Tyrosyl-DNA phosphodiesterase 2 (TDP2) {also known as TRAF and TNF receptor-associated gene (TTRAP) or ETS1-associated protein II (EAPII) } is a 5′-tyrosyl DNA phosphodiesterase that can remove the covalently-attached abortive complexes generated by DNA topoisomerase II (TOP2) when it is unable to complete its normal catalytic cycle. Fortunately, this type of DNA lesion is efficiently repaired, in part though the action of TDP2, which hydrolyses the phosphotyrosyl bond in a magnesium cofactor-dependent reaction, leaving ligatable 5′-phosphate moieties. Consequently, TDP2 has attracted interest as a target for small molecule inhibitors that might have utility in overcoming innate or acquired resistance to TOP2 poisons. Using a ‘humanized’ mouse TDP2 expression construct, we have now determined X-ray crystal structures of the catalytic domain of TDP2 in complex with deazaflavin inhibitors, revealing the unusual molecular interactions underpinning their mode of action.

We therefore created the expression construct m2hTDP2CAT (m2h=mouse-‘to’-human) by mutating the following mouse residues to their human equivalent: E242G, Q278R, Y321C and H323L. We were successful in obtaining diffracting crystals of 148 in complex with m2hTDP2CAT, determining the structure at a resolution of 1.7 Å. In this instance, we also supplemented the purification buffers with manganese chloride (iso-structural with magnesium, but readily discernible in electron density maps) in order to more fully define any interaction of the inhibitors with the metal-dependent catalytic centre of the enzyme. In the 148 complex, the side chains of Arg276 and Asp277 make the same set of interactions with the carbonyl and nitrogen groups of the pyrimido-dione ring, as with 163. However, the side chain of Arg241 occupies a different position, breaking its hydrogen bond interaction with Asp277, and instead packing in a π–π interaction against the face of the tricyclic core of the deazaflavin. Interestingly, the p-hydroxyl group of the R1 substituent in 148, points directly towards the catalytic core of the protein and makes a series of water-mediated contacts to the side chains of Asp272 and Asn274. Electron density maps also clearly showed the position of a tartrate molecule (picked up from the crystallization mother liquor), which is hydrogen-bonded to the side chain of Ser239, as well as an extensive series of water-mediated interactions with several amino acid residues surrounding the catalytic centre. The tartrate molecule also completes the octahedral coordination of the Mn2+ ion (marking the position of the catalytic Mg2+ cofactor). Moreover, its position marks a potentially useful ‘molecular interaction path’ that could be utilized in future iterations of TDP2 inhibitor compounds.

>[2x]SNALEDSSTISFITWNIDGLDGCNLPERARGVCSCLALYSPDVVFLQEVIPPYCAYLKKRAASYTIITGNEEGYFTAILLKKGRVKFKSQEIIPFPNTKMMRNLLCVNVSLGGNEFCLMTSHLESTRGHSAERIRQLKTVLGKMQEAPDSTTVIFAGDTNLRDREVIKCGGLPDNVFDAWEFLGKPKHCQYTWDTKANNNLRIPAACKLRFDRIFFRAEEGHLIPQSLDLVGLEKLDCGRFPSDHWGLLCTLNVVL>[2x]GSHMGSQFWVTSQKTEASERCGLQGSYILRVEAEKLTLLTLGAQSQILEPLLFWPYTLLRRYGRDKVMFSFEAGRRCPSGPGTFTFQTSQGNDIFQA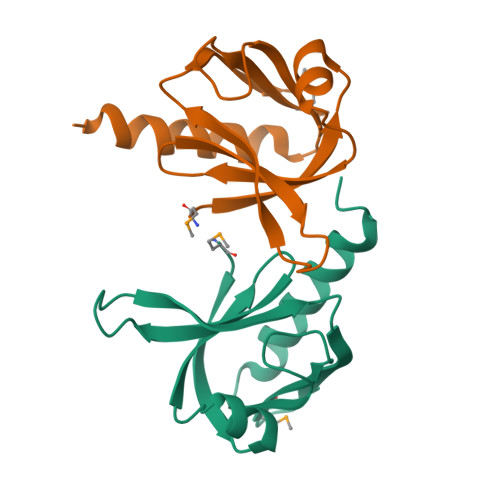VEAAIQQQKAQGKVGQAQDILRLEHHHHHH>MWRYESVVGGCSFMGGEVEEPEPQMVLSPLTSAAIFLVVTIDSGGEDTVRDLLSDVASLERAVGFRAQPDGRLSCVTGIGSEAWDRLFSGARPAGLHPFRELDGPVHRAVATPGDLLFHIRASRLDLCFALATEIMGRLRGAVTPQDEVHGFKYFDERDMLGFVDGTENPTGAAARRAVLVGAEDPAFAGGSYAVVQKYLHDIDAWEGLSVEAQERVIGRRKMTDVELSDDVKPADSHVALTSVTGPDGSDLEILRDNMPFGSVGREEFGTYFIGYARTPEVTETMLERMFLGTASAPHDRILDFSTAVTGSLFFTPAADFLEDLSARP[6x]

A widely applicable approach is the use of photocaged substrates, where the photocage is soaked into the crystal in advance and then activated using a laser pulse to provide uniform initiation of the reaction throughout the crystal. This work characterizes photocage release of nitric oxide and binding of this ligand to two heme protein systems, cytochrome c′-β and dye-decolourizing peroxidase B using a fixed target sample delivery system. In this work, we describe a thorough characterization of the application of the NO photocage N,N′-bis-(carb­oxy­methyl)-N,N′-di­nitroso-1,4-phenyl­enedi­amine (henceforth referred to as NO cage) to room-temperature microcrystals of two proteins: a gas binding cytochrome c′ (McCP-β) and a dye-decolourizing peroxidase B (DtpB). Laser parameters for photoactivation are systematically explored, and time-resolved structures over timescales ranging from 100 µs to 1.4 s using synchrotron and XFEL beamlines are described. We have demonstrated a sample and time efficient approach using fixed targets to carry out time-resolved SSX and SFX experiments with an NO photocage over the microsecond to second time regimes.

On binding to the heme, NO was observed to bind in an end-on fashion via the nitro­gen atom with an Fe—N distance of approximately 2.0–2.5 Å and an Fe—N—O angle of approximately 105–150°. The variability in these values occurs across the six independent heme groups within the crystallographic model and could represent either genuine differences in binding due to subtle differences in the crystalline environments or simply uncertainty in modelling a small ligand into the electron density features. A small shift in the side-chain position of Asn245 was observed compared with the ‘empty’ site structure in all six of the hemes, and at all laser powers and timepoints. An intriguing observation was that of differing occupancies for the released NO within the different (chemically identical) monomers of the homo-oligomeric proteins, particularly for the hexameric DtpB (in contrast, McCP-β is a homodimer). One possible explanation would be differences in the proximity to the bulk solvent channels in which the photocage molecules presumably are present, although no correlation was seen between chains with higher NO occupancy between the differing laser powers. Assessment of occupancies in light-activated processes remains challenging, particularly for small ligands such as the diatomic NO. For our experiments with DtpB, we found both B-factor and Fo − Fc peak height quantification to give results that display the same occupancy trend with laser power, but both generally overestimate NO occupancy compared with multicopy refinement [Fig. 6(f) and Table S4].>[2x]ADQRRDFIDIESKFALRTPEDTAEDTCHLIPGVAESVATCHFNHSSKTFMVIHGWTVTGMYESWVPKLVAALYKREPDSNVIVVDWLSRAQEHYPVSAGYTKLVGQDVARFINWMEEEFNYPLDNVHLLGYSLGAHAAGIAGSLTNKKVNRITGLDPAGPNFEYAEAPSRLSPDDADFVDVLHTFTRGSPGRSIGIQKPVGHVDIYPNGGTFQPGCNIGEAIRVIAERGLGDVDQLVKCSHERSIHLFIDSLLNEENPSKAYRCSSKEAFEKGLCLSCRKNRCNNLGYEINKVRAKASSKMYLKTRSQMPYKVFHYQVKIHFSGTESETHTNQAFEISLYGTVAESENIPFTLPEVSTNK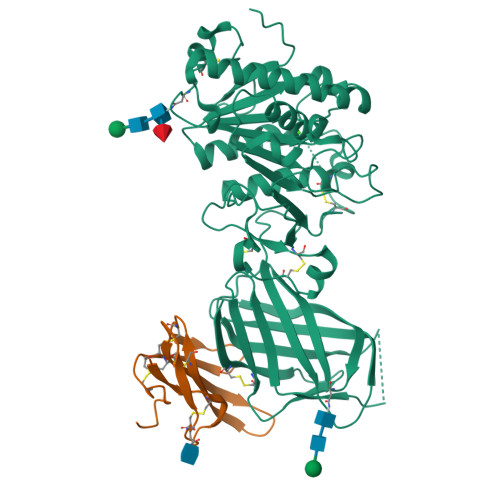TYSFLIYTEVDIGELLMLKLKWKSDSYFSWSDWWSSPGFAIQKIRVKAGETQKKVIFCSREKVSHLQKGKAPAVFVKCHDKSLNKKSG;>QTQQEEEEEDEDHGPDDYDEEDEDEVEEEETNRLPGGRSRVLLRCYTCKSLPRDERCNLTQNCSHGQTCTTLIAHGNTESGLLTTHSTWCTDSCQPITKTVEGTQVTMTCCQSSLCNVPPWQSSRVQDPTG[2x]>[2x]GHMIKICIAGKNNIAVNSLQFILKNYFEADQIVVIPNKNDKGIDSWQKSLLKFALDNNIKIVTLDEIYNIE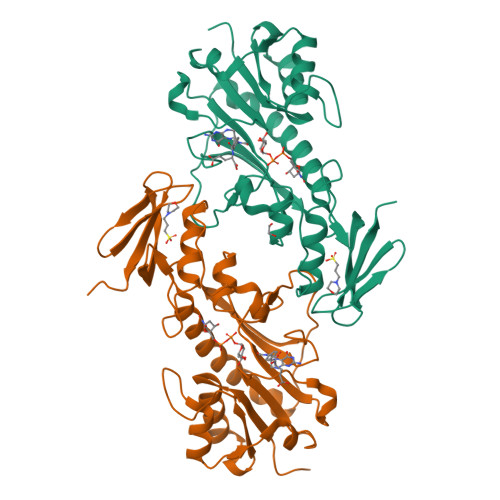QIIFFSLEFDQIIKIENFKSDRLFNIHFSALPKYKGVFTSITPILNNELESGVTLHRIDNGIDTGNIIDQHCFPIDINDTARDLYFNYLKYGESIFKKNIQTIINNSYKDLKQTNINSSYFSRKDINLVHKINFKKTSFEIHNQIRAFIFQEYQLPIINNSKIIKSILANEFIGYNVFEEFENYFIISGIDGFKIIAQKLNKL> RA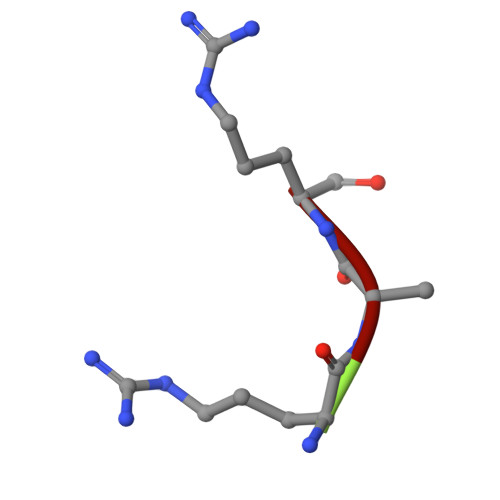R> MIGRLRGIIIEKQPPLVLIEVGGVGYEVHMPMTCFYELPEAGQEAIVFTHFVVREDAQLLYGFNNKQERTLFKELIKTNGVGPKLALAILSGMSAQQFVNAVEREEVGALVKLPGIGKKTAERLIVEMKDRFKGLHGDLFTPAADL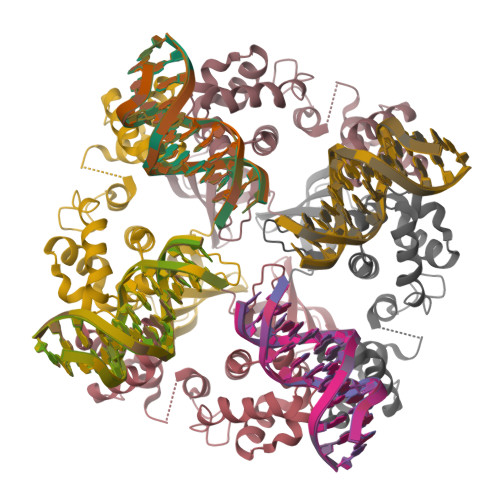VLTSPASPATDDAEQEAVAALVALGYKPQEASRMVSKIARPDASSETLIREALRAAL> MNVGVNWSGQRELPCINQLFLTRDIDFVELLIDNFLTTDVDSIKAFLAGRPCAFHIMNSQFLHKDERELLAMAKIINKLIHSLQPIYISDHIGKFYHRGQALPQMLEVDYGLQTHSTIKKVKAWSSLLDGKLLLENYPSIFPQDMSQIDFFKRILEETYCGLLFDISNAFIAEVNIKQSRTSWFDLIKHCQHFHIAGFENAPDNQFLVDTHSQCIEEPVLSFLQEVNNATSIATISVERDENFDVSDWALDIDNVRNRVS;> MNVGINWSGQRELPCINQLFLTRDIDFVELLIDNFLTTDVDSIKAFLAGRPCAFHIMNSQFLHKDERELLAMAKIINKLIHSLQPIYISDHIGKFYHRGQALPQMLEVDYGLQTHSTIKKVKAWSSLLDGKLLLENYPSIFPQDMSQIDFFKRILEETYCGLLFDISNAFIAEVNIKQ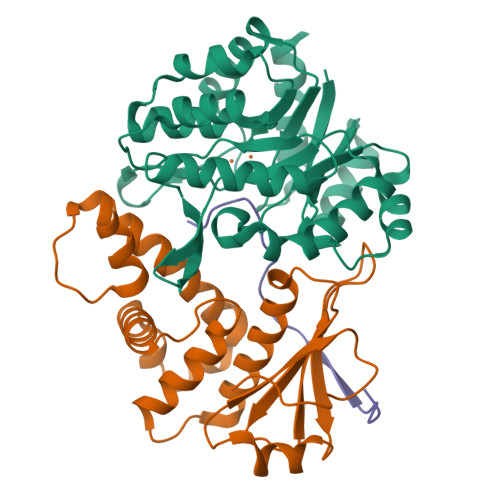SRTSWFDLIKHCQHFHIAGFENAPDNQFLVDTHSQCIEEPVLSFLQEVNNATSIATISVERDENFDVSDWALDIDNVRNRVS;>[2x]MEEILDRIINPLSAKPLTKKEHIYTSLVLQSSQSLILSACPSLQSQRQFCSFEYHQQFIDWCFFNKKRTDWCLALSFYQYLSYKNEQVSVEILKELIHLACSQWTYADKSTNQTVVICHTRLPSMVFGGNKSLFAQEFREVFLLETEQLKPFIQSHVPDGYFVYWILRDDSEYPSTMGEK;> MKNDKKVVVKVKDKEMTCGAFNK;> MKNDKKVVVKVKDKEMTCGAFN>MKNLSAYEVYESPKTSGESRTEAVSEAAFESDPEVSAILVLTSSEASTLERVADLVTAHALYAAHDFCAQAQLAAAELPSRVVARLQEFAWGDMNEGHLLIKGLPQVRSLPPTPTSNVHAVAATTPMSRYQALINECVGRMIAYEAEGHGHTFQDMVPSAMSAHSQTSLGSAVELELHTEQAFSPLRPDFVSLACLRGDPRALTYLFSARQLVATLTTQEIAMLREPMWTTTVDESFLAEGRTFLLGFERGPIPILSGADDDPFIVFDQDLMRGISAPAQELQQTVIRAYYAERVSHCLAPGEMLLIDNRRAVHGRSIFAPRFDGADRFLSRSFIVADGSRSRHARSSFGRVVSARFS[4x]

We have focused our work on the iron(II)/α-KetoAcid-dependent Oxygenases (αKAOs), a mechanistically diverse superfamily of enzymes that use dioxygen as the oxidant to catalyze several reactions via C-H bond activation, mostly hydroxylation. These enzymes operate with three substrates, dioxygen, α-ketoglutarate (α-KG) and a primary substrate. One of these, KDO1, catalyzes the formation of (3S)-3-hydroxy-L-lysine, while five others, KDO2 to KDO6, promote the formation of (4R)-4-hydroxy-L-lysine. We based our analysis on the structures that we solved by X-ray crystallography of two of the regiodivergent αKAOs active towards L-lysine, namely KDO1 from Catenulispora acidiphila, that catalyzes the C-3 hydroxylation, and KDO5, from Flavobacterium sp., that catalyzes the C-4 hydroxylation.

In KDO1, the L-lysine complex shows a well ordered lysine in monomer C. The interacting residues are Glu180, Arg332, Asp 234, Asp 268 (salt bridges 2.9 Å; 3.0 Å and 3.0 Å; 2.9 Å; 2.7 Å), Ser168 and Ser236 (H-bonds 3.2 Å and 3.3 Å; 3.3 Å). The Nε is restrained at the bottom of the pocket by two salt bridges with the Oδ2 of Asp268 and the Oδ1 of Asp234, while in KDO5 the Nε is stabilized via a water molecule in interaction with Asp260. The size of the KDO1 pocket is smaller than that of KDO5 due to Ser168 (instead of Gly). For KDO1, the adjacent loop has a direct impact on positioning the substrate in the active site as Ser168 (P6 in the logo) makes a H-bond with the carboxylate group of the lysine. In the closed form, the lysine or hydroxy-lysine/succinate are covered by the adjacent loop and the active site is locked by interactions between Thr167 (P5) and Ser236 (P14). In the absence of the α-KG, unlike what is observed for the lysine-KDO1 complexes, the lysine is positioned differently in the four molecules of lysine-KDO5, suggesting that this substrate is not properly stabilized.>PVPNPTMPVKGAGTTLWVYKGSGDPYANPLSDVDWSRLAKVKDLTPGELTAESYDDSYLDDEDADWTATGQGQKSAGDTS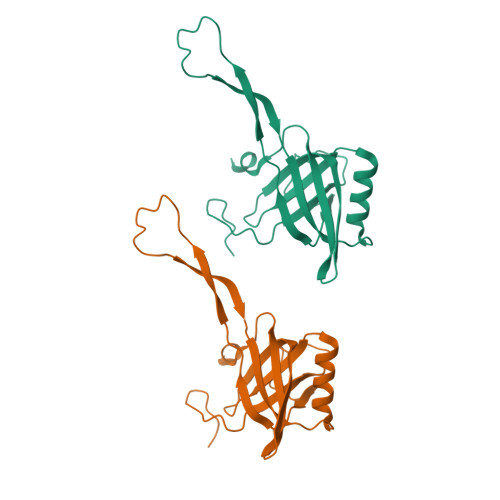FTLAWMPGEQGQQALLAWFNEGDTRAYKIRFPNGTVDVFRGWVSSIGKAVTAKEVITRTVKVTNVGRPSMAEDRST[2x]> GSHMGKRVLIVDDAAFMRMMLKDIITKAGYEVAGEATNGREAVEKYKELKPDIVTMDITMPEMNGIDAIKEIMKIDPNAKIIVCSAMGQQAMVIEAIKAGAKDFIVKPFQPSRV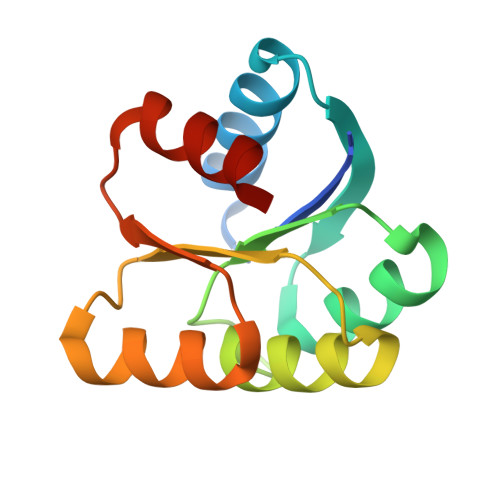VEALNKVSK> MQVESLQNLQVKIRNDERNHSLTKKYLTDDIVKKYQATKTSLGGTLAQCVNTNAYNPGALLPRSCDLNAYETFRDFFDAVIADYHKVPDGKIQHPKSNFGDLKSLSFTDLNTYGNLVVSTRVRLGRTVEGFGFGPTLTKETRIELENKISTALHNLSGEYEGTYYPLTGMSEEDRIKLVNDHFLFRNDDNVLRDAGGYIDWPTGRGIFINKQKNFLVWINEEDHIRVISMQKGGGLTAVYKRLADAIQELSKSLKFAFNDRLGFITFCPSNLGTTLRASVHAKIPMLASLPNFKEICEKHGIQPRGTHGEHTESVGGIYDLSNKRRLGLTELDAVTEMHSGVRALLELEVMLQEYNKGAPEGVMPVEPLTYLAKLLEGASIEKCYTRKYLTPEIIKKYDGKRTTHGATLAHMIRNGAYNNRSICPRTGEAECYSTFIDYLDPLICDYHGVKDSAFKHPAPTFGDLSKLPFGDLDPTGKFIVSTRVRVGRSVEGFLFPTIMSKTDRIKLEQVISGALKGLTGEHAGTYYPLTDMKEEDRKQLVEDHFLFKNDDPVLRDAGGYRDWPVGRGIFHNNSKTFLVWVCEEDHM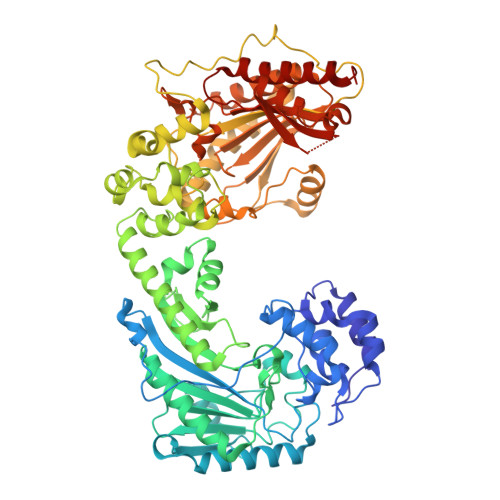RIISMQQGGNLAAVYKRLIEGINAIGKSMKFAHSDKYGYITCCPSNLGTSMRASVLLKIPKLSSQPKKLDEICAKYMLQARGLYGEHTESPDGTYDISNKRRLGLTELQAAHEMAEGVAKMIEIEKGL>[8x]SAAATQAVPAPNQQPEVFCNQIFINNEWHDAVSRKTFPTVNPSTGEVICQVAEGDKEDVDKAVKAARAAFQLGSPWRRMDASHRGRLLNRLADLI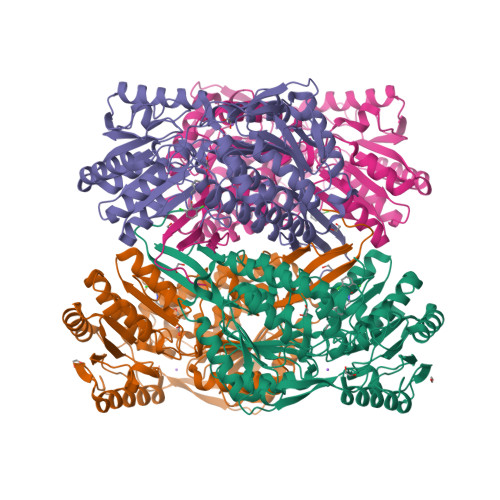ERDRTYLAALETLDNGKPYVISYLVDLDMVLKCLRYYAGWADKYHGKTIPIDGDFFSYTRHEPVGVCGQIIPWNFPLLMQAWKLGPALATGNVVVMKVAEQTPLTALYVANLIKEAGFPPGVVNIVPGFGPTAGAAIASHEDVDKVAFTGSTEIGRVIQVAAGSSNLKRVTLELGGKSPNIIMSDADMDWAVEQAHFALFFNQGQCSCAGSRTFVQEDIYDEFVERSVARAKSRVVGNPFDSKTEQGPQVDETQFKKILGYINTGKQEGAKLLCGGGIAADRGYFIQPTVFGDVQDGMTIAKEEIFGPVMQILKFKTIEEVVGRANNSTYGLAAAVFTKDLDKANYLSQALQAGTVWVNCYDVFGAQSPFGGYKMSGSGRELGEYGLQAYTKVKTVTVKVPQKNS> QQVCTQQAETHPPLTWQKCTASGCTPQQGSVVLDANWRWTHDTKSTTNCYDGNTWSSTLCPDDATCAKNCCLDGANYSGTYGVTTSGDALTLQFVTASNVGSRLYLMANDSTYQEFTLSGNEFSFDVDVSQLPCGLNGALYFVSMDADGGQSKYPGNAAGAKYGTGYCDSQCPRDLKFINGQANVEGWEPSSNNANTGVGGHGSCCSEMDIWEANSISEALTPHPCETVGQTMCSGDSCGGTYSNDRYGGTCDPDGCDWN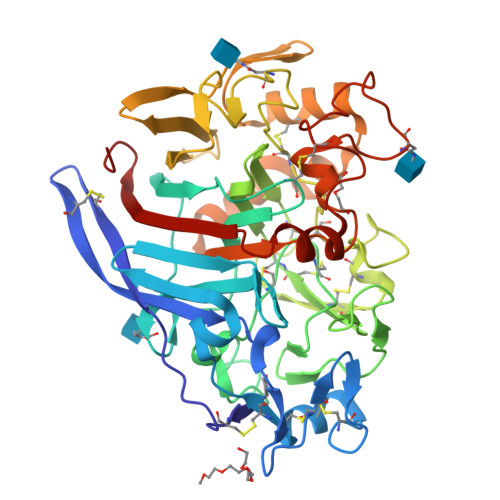PYRLGNTSFYGPGSSFALDTTKKLTVVTQFATDGSISRYYVQNGVKFQQPNAQVGSYSGNTINTDYCAAEQTAFGGTSFTDKGGLAQINKAFQGGMVLVMSLWDDYAVNMLWLDSTYPTNATASTPGAKRGSCSTSSGVPAQVEAQSPNSKVIYSNIRFGPIGSTG> 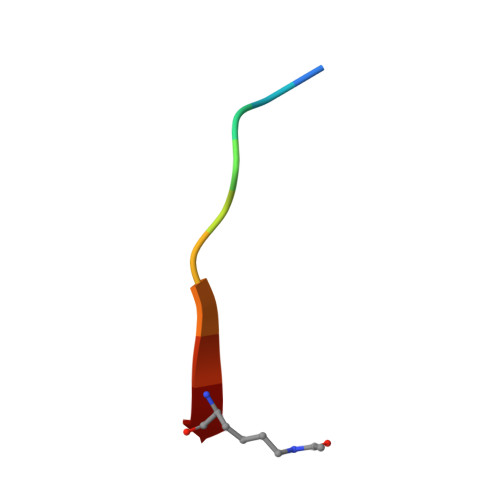EDQHTQITKV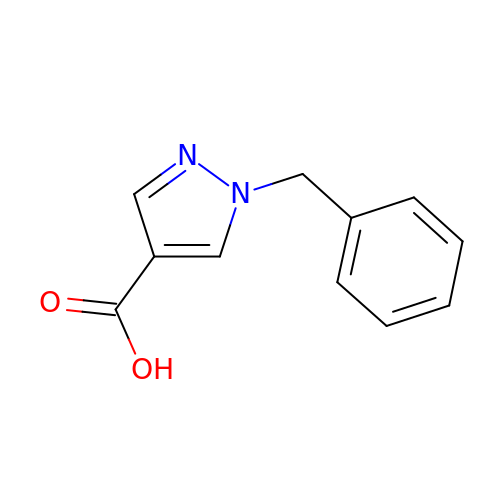1-benzyl-1H-pyrazole-4-carboxylic acid | C11 H10 N2 O2 | KGDOHXYALMXHLF-UHFFFAOYSA-N CE2 enzymes are acetyl esterases (that are generally not appended to other catalytic modules), which are reported to be active on synthetic aryl-esters and acetylated xylan. Here we report the biochemical properties and crystal structure of several CE2 members, both single-module CE2 enzymes and CtCE2, a component of CtCel5C-CE2. All three 3D structures reveal a bi-domain enzyme in which an N-terminal β-sheet “jelly roll” domain (around 130 residues) is linked to a C-terminal domain of approximately 220 residues. The C-terminal domains possess an atypical α/β-hydrolase (SGNH-hydrolase) fold, consisting of repeating β-α-β motifs that form a curved central five-stranded parallel β-sheet, in the strand order β2, β1, β3, β4, and β5 with strand β2 interrupted by loop insertion.

The structure of both wild-type CtCE2 and the S612A mutant were determined in the presence of cellohexaose and clear electron density for five β-1,4-linked d-glucose molecules was observed in the cleft, consistent with the affinities revealed by ITC. Notably, the O6 of Glc-4 makes a hydrogen bond with Oγ of Ser-612 (in one of its two conformations) in the wild-type esterase and Nɛ2 of His-791 in the S612A mutant, while O6 of Glc-2 interacts with Oɛ1 of Gln-780. Mutation of His-791 to alanine reduces affinity for cellohexaose ∼20-fold but, intriguingly, the S612A mutant binds to the oligosaccharide ∼8-fold more tightly than the native protein. In the wild type enzyme Ser-612 adopts two conformations. In one conformation the hydroxyl makes a polar contact with cellohexaose forcing the ligand away from the histidine. In the S612A mutant the hexasaccharide adopts a different conformation in which it is now able to make a, presumably more productive, hydrogen bond with the histidine. Indeed, the bond distance between Ser-612 and Glc-4 is 3.3 Å (the two conformations adopted by the serine suggests a relatively weak interaction with the glucose), while the bond distance between His-791 and Glc-4 is reduced to 2.8 Å, pointing to a stronger interaction. Indeed, the kinetics of inhibition are consistent with the observation that cellohexaose binds more tightly to the enzyme when it makes a polar contact with His-791 rather than Ser-612; when the serine is in complex with acetate (or formate in the crystal structure) it is not available to hydrogen bond with the hexasaccharide that is now able to interact with His-791.

> MASPDEDNPGILYNGRFDFSDPNGPKCAWSGSNVELNFYGTEASVTIKSGGENWFQAIVDGNPLPPFSVNATTSTVKLVSGLAEGAHHLVLWKRTEASLGEVQFLGFDFGSGKLLAAPKPLERKIEFIGDAITCAYGNEGTSKEQSFTPKNENSYMSYAAITARNLNASANMIAWSGIGLTMNYGGAPGPLIMDRYPYTLPYSGVRWDFSKYVPQVVVINLGTNDFSTSFADKTKFVTAYKNLISEVRRNYPDAHIFCCVGPMLWGTGLDLCRSYVTEVVNDCNRSGDLKVYFVEFPQQDGSTGYGEDWHPSIATHQLMAERLTAEIKNKLGWLEHHHHHH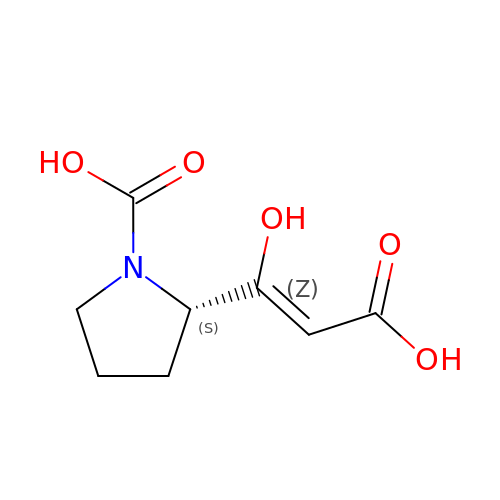(2S)-2-[(Z)-1,3-bis(oxidanyl)-3-oxidanylidene-prop-1-enyl]pyrrolidine-1-carboxylic acid | C8 H11 N O5 | ROSCYVZNGZEOEY-YIWIKUPCSA-N> SNAQQVTVEDHQSTPVHIKLQPPVTIESFVRRGEPFESTYTAVPERVVAMWQNSIE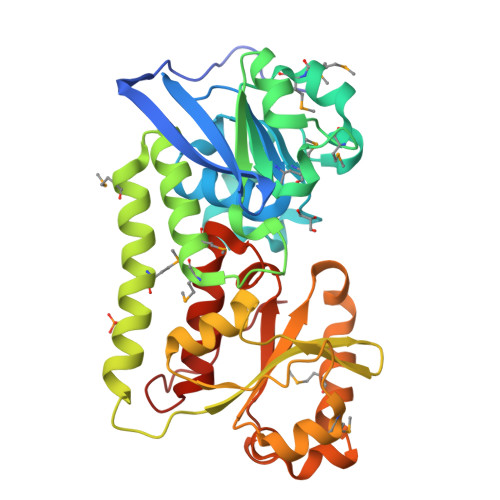TIIALGEGDRIVAGMGIPDRKYVRPEYREAYDKIPYKDLKYANLESVLMMKPDLLVGWKSTFTNKMLQTPTFWQARLANVYIAESSLGAQSALTMDMEYKYIRDLGRIFNRNMEAERLIQEMQQSVAYTVAQTAHEKPPKALFIEVQGKHFRLYGHKTLAGNIGASLHADVIDTETPSISMEDVVEQNPDVIFLIVSDGEYSQADVIMNYVLTQSGLQGVNALRNKRVHFLPLLAVYSPGIRLLDSIDIVSHGLYPNLYPEGVPDLIH> MEELFNALPQPLQQLSLALAGEIPLTDHIFEQAASTWHVQPRSLTYKLLDHIPFATPVVVPPSIYHSLDWSKCFAVNQDRVERIPTIDNPDDVYVPNSDIGPLLTSLHTIPDYGFLHPTIENDATTLRAERARCASTFYKIASSQARQVKLDPIRMLGFLLLVQARPRVPSGLVTDQPTRRDPTLSPALHAIWQVMQYYKVAGVYYAPALVVPSGAIWWIPPPGKRNVVSVQYLLTDLISLAILAHMTDMSPTLELTGVLMYLRAASSHSYAYTLLQMKSVFPALSLRSMYRNKGFGGKAPAIEWTEPRSKYKFRWTGVTQLHDGLRPRSPSMDVPTLETLAKYELVDIGHTIIRERNAHPQHNHDSVRFVRDVMALTSGMYLVRQPTMSVLREYSQVPDIKDPIPPSAWTGPIGNVRYLLPSVQGPARHLYDTWRAAARQIAQDPQWHDPLNQAIMRAQYVTARGGSSASLKFALKVTGIVLPEYDDSKVKKSSKIYQAAQIARIAFMLLIAAIHAEVTMGIRNQVQRRARSIMPLNVIQQAISAPHTLVANYINKHMNLSTTSGSVVTDKVIPLILYASTPPNTVVNVDIKACDASITYNYFLSVICGAMHEGFEVGNADAAFMGVPSTIVSDRRSPVAPYSRPISGLQTMVQHLADLYAAGFRYSVSDAFSSGNKFSFPTSTFPSGSTATSTEHTANNSTMMEYFLNVHAPSHVKSASLKRILTDMTIQRNYVCQGDDGILLLPHEAASKISADDMNELLTCLRDYGQLFGWNYDIDWSDTAEYLKLYALMGCRIPNTSRHPPVGKEYAAPQTDEIWPSLIDIVIGHHLNGVTDVLNWREWLRFSWAFACYSSRGGYTNPRGQSFSAQYPWWTFVYLGIPPILLPGQTPFIHSCYMPPGDQGMFSILNGWRDWLISHASTTLPPLRHNHPVWGLSDVPSLLSQFGVYAGYHAAQHYRRPKPAPETASSDSINQITSDLTEYLFYDSALKARVMKGRYNWERLSSSLSLNVGSRVPSLFDVPGKWVAAGRDAEKPPPSSVEDMFTSLNRCIRRPTHSFSRLLELYLRVHVALGESIPLAIDPDVPQVAGADPANDDHWFKYTCLGDIPSATRNYFGESLFVGRVVSGLDVEAVDATLLRLKILGAPPEAFIAVLNGIGMSDSEAHQIAGRISLANAQLVQIARVVHLSIPSSWMTLNTGPYIHHHAYDFKPGITQPSAKSRDKSIWMSPILKLLCTSYAMTVAGPVRTSIVTEIDGSAAALSGNLRVWMRDV;> MITIVVIPTAHFSWTDTNFLNSVDYRLTSQPKIRDRFAVYAPGWLRRQLDEFSASLTASELLQALQTIPIPVKARCLLLPKPKRFAQWLLDVPSANIWHIPVTTLRATVASKHPSSDVYNYIPDHVPPNAEFDTVTRRVAAGRDIYVRSTKVIGAPLCLAAPAKYYAGYLSTHQLDGIYPENWAPDNFHKREFCLTILPSLLGPRTFLLDVDADRDASYPLSVLWPQLRALALKSRLLLPPVALLRRVVDPGLKPTWSADSDAAFRALRLSRPSSASKPVGFDFSALPVVDIICLLESEPDDHGRIAPGTRLTIHSVPTDLLTSLSIQEGVRYPLRQESGMFVHWVLLALLMSDDVTISGTRRSVKLETAHASARPFVHITVERCASARIIDVRGSPAMYANAVCLTLPKGSYKSTIIDTLPAMFSDLPILEQAAVIDSDALGDSLRPSFETQFLERLENLDPNLLDRAVASILSPTSDTSDDAVTTVLDAFNALYREIMTPAQRARLPLLTQQGRVLAFAHSDYELLSANIPIQVVRGSIPIDHVVNLLARRNRVGGTALQVLLDYCYRTQASPLAPTPAGRLYKQLFGPWLMVPRLSEPLIKLRLVASAPAKVLRAAGWTIDGDPPLEVSCLCAYVTDRAAATALIERRLDSRALVTVGGDQLMFVEYAPPLPLVSIPRTFLLPVTYVVHWVPPQRVLLNGGNVSFTSGLEWTFDDDPQVVTSTGV;>MPRRSARKAQSAIASPADTNVVPAKDAPTTNSPPSTTSPNQAAADANQQQAGIVSSQSGPNAVGDSAPSSSVNNDGDIITRPTSDSIAAVANATKPAAVVSDPQSMKVTPIVNPSSYVCNVCNARFSTMSALSEHLRSDHRDDASTLLATPMINNAIRSFLTAWDDIRILSPDVSSKSLSAYLDSAVANGPELIIEDTGLCTSFMLLDNIPSAHLTKELIGFTWFMQMYQMTPPLPEGAVNRIVCMTNWASLGDEGRGLEVRLPPPTDSSVHAYKTVLSRGYIDNAQFNPLALRSNVLLMLLQFTLSNLKINKSSTFTSDVTTITSGRMIRAFEGRPELLALAYPGRAVLPTQTKNAQFLSTAIADRIGRLDRANLIGGEVSAMVECMELCDALTLHIRETYIMLLRSMHQDPTQIVQIVNECANNLLNSTIPISLRPTILCPWFASSEDLRLQQVMHLVNISSNTAAALPLVEALSTLLRSVTPLVLDPTVLTNAITTISESTTQTISPISEILRLLQPMGNDYAAFWKCIASWAYNGLVTTVLSEDAFPDSSQSITHLPSMWKCLFLTLAGPMTSDPHSPVKVFMALANLLAQPEPIAIGVPGMHQTTPASQFSHPGVWPPGFLNPQLINPQQAPLLRAFAEHIRANWPQPSEFGYGSTLQGSANLFIPSNRMVYPWPNQPLPRLTVAPTYDSAMSNWISTTIAFFIRVVNSVNMTATVNDLTRRTMTGVMTAMRQVKTMTPF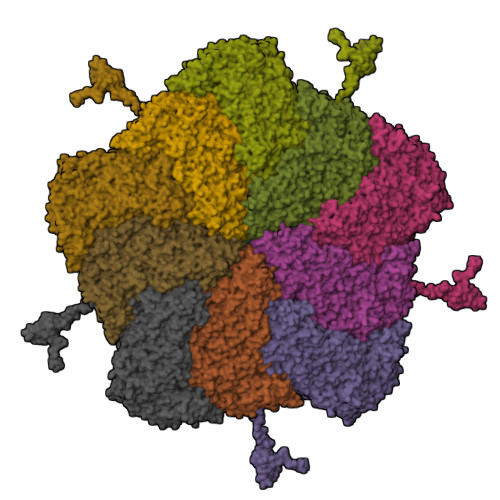YIQHMCPTELSVLASVTVTPPFQVPFTRLVQNDVITNVLVARVDPAQRGDAAVDIRATHATFAAALPVDPAAIVVAMLCGQTETNLIPSHHYGKAFAPLFASNAMFTRNQRAVITREAFVCARSAVAQCQDAGFLVPRPLDALRQFDVTSAAAAEIMHAVNDAFKTAFDLDGALLDGLALYGDPRIADLSAAYLQYGGNVVREHVPPGPSHIHRALQQVESTFMAEMNLFNVARGNLYLVQTATNGNWSPMAPVAAPPFVRGGPNVRVVGRFGTIVPRPNGLEPQLIDDGNVPRDIAGDWVYPSDVLQVSVAVFRDYVWPMVKAGRTRVLVELGHYVYTLHYYDPQISLDEAPILEEWLSKINPAGIPPVPFCIPIPQVYPCITARRVHYAFTSENNNDSLFSTNAASIDTAFGENAAVSPLRWPGLVDPNYRVGTNDLPNRITLYNSLYRYNFTYPTLDGIMYVRSAT[10x]>MAHHHHHHMKTKDAVAVVTGGASGLGLATTKRLLDAGAQVVVVDLRGDDVVGGLGDRARFAQADVTDEAAVSNALELADSLGPVRVVVNCAGTGNAIRVLSRDGVFPLAAFRKIVDINLVGTFNVLRLGAERIAKTEPIGEERGVIINTASVAAFD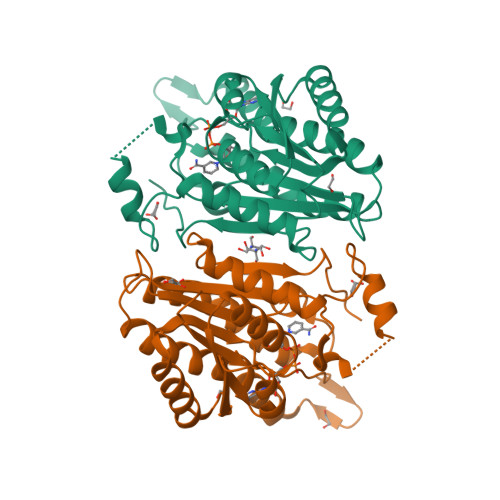GQIGQAAYSASKGGVVGMTLPIARDLASKLIRVVTIAPGLFDTPLLASLPAEAKASLGQQVPHPSRLGNPDEYGALVLHIIENPMLNGEVIRLDGAIRMAPR[2x]>MSEGEGQAKNRLFLGIDLGTSHTAVMSSRGKKFLLKSVVGYPKDVIGLKLLGRPYVVGDEAFEMRSYLDIRYPLQDGVLSEISDRDIEVARHLLTHVVKSAEPGPNDEICAVIGVPARASAANKALLLKMAQEVVHTALVVSEPFMVGYGLDKLINTIIVDIGAGTTDICALKGTVPGPEDQVTLTKAGNYVDERLQNAILERHPELQMNVNVACAVKEQFSFVGTPTEVASFEFRAAGKPVRADVTEPVKIACEALMPDIIESIETLLRSFQPEYQATVLQNIVFAGGGSRIRGLAAYVKEKLRPFGDANVTCVKDPTFDGCRGALRLAEELPPQYWRQLGD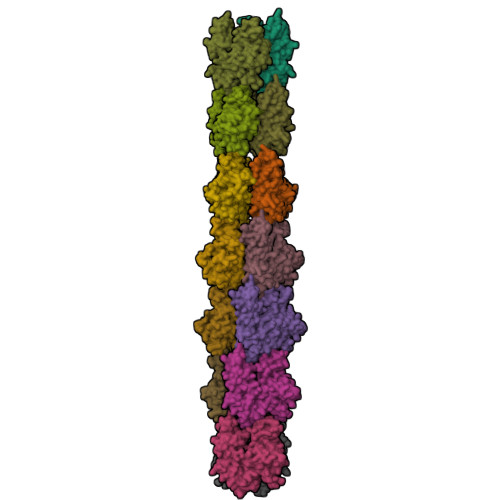VSGS[14x]> MATFPGFQVPKPVEGIVAGITPNIDALELNQDISLAAVAASTWGGAYGAHQPVEVIHSTYQAVHQSALEENYYNRLWLIPTAMELGNVVSTQIRPASVWNAYFSPRTLTAIDREAADGITLSGQASPPLGFAALEERTWTVSIGTDGPPVVNARIVWRLQGEPNLVLVITGNRIIAWTFAPDWGDSIVERLSASTNILQSESAVTQRRAMRLAPRREFDANMYA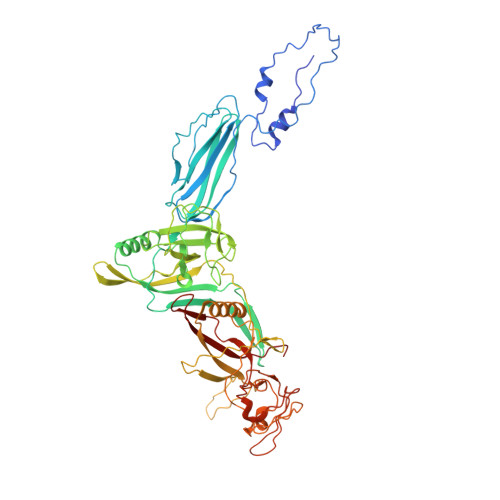VDRERQLLDMTLFGWGARIWALPIWPDIQLLHQPLAAGSLGIPCDTAGLDFRDGGLAMLRGEDAFTYEVVEVKTVTASGLDLVRPVQAAWGTGSRLYPVRTAQLTEQPTLTRLTDTAQSARVSFLVMEPSAWPELMPATTYRGRPVLEQRPDESEDLTSSYQRLLSTLDNGSAIPRVTDVAGMALPVIGHRWIGMGRAERSAFRSLVYALRGQQKPLWVPTHADDLTLVATVSQLSTALDVRNIGYARFANGRPGRRDIRIELYDGTVYHRRILTSTELDADTERVAIDAALGRLVEPTDVARICFMALCSAASDVVEIEHVTDSEGVATAALTFKGVRDDEF> DIKVTPG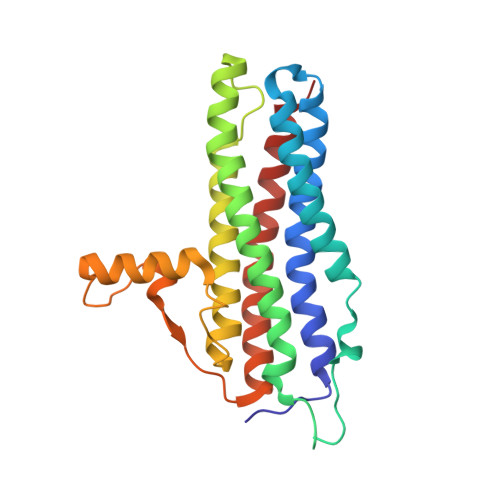TSELVEQILALLSRYLSSYIHVLNKFISHLRRVATLRFERTTLIKFVKKLRFYNDSVLSYNASEFINEGKNELDPGADSFDKVILPIASMFVKCVETFDLLNYYLTQSLQKEILSKTLNEDLTLTAESILAIDDTYNHFVKFSQWMIESLRIGSNLLDLEVVQFAIKSADEDGTNIGETDNIFLQEILPVNSEEEFQTLSAAWHSILDGKLGALDEEFDVVATKWHD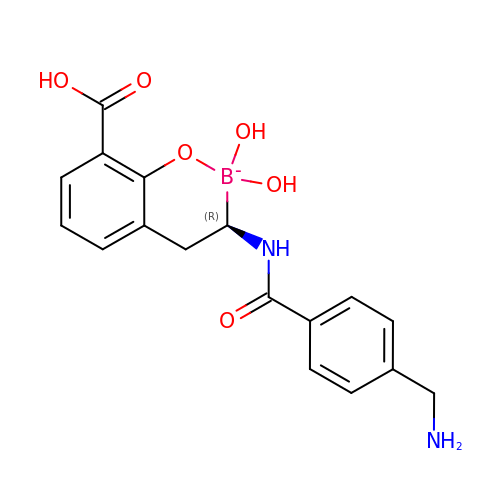(4~{R})-4-[[4-(aminomethyl)phenyl]carbonylamino]-3,3-bis(oxidanyl)-2-oxa-3-boranuidabicyclo[4.4.0]deca-1(10),6,8-triene-10-carboxylic acid | C17 H18 B N2 O6 | QLXKUYDHLJOWQG-AWEZNQCLSA-N> MPLLTQQIQ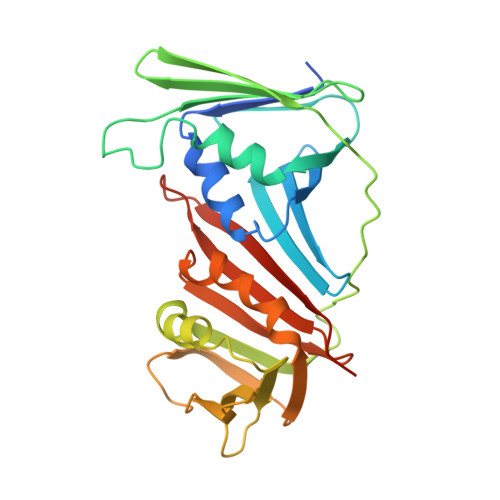DEDDQYSLVASLDNVRNLSTILKAIHFREHATCFATKNGIKVTVENAKCVQANAFIQAGIFQEFKVQEESVTFRINLTVLLDCLSIFGSSPMPGTLTALRMCYQGYGYPLMLFLEEGGVVTVCKINTQEPEETLDFDFCSTNVINKIILQSEGLREAFSELDMTSEVLQITMSPDKPYFRLSTFGNAGSSHLDYPKDSDLMEAFHCNQTQVNRYKISLLKPSTKALVLSCKVSIRTDNRGFLSLQYMIRNEDGQICFVEYYCCPDEEVPESES>MNFPQLSKEVAEDEAEVILHTSQGDIRIKLFPKLAPLAVENFLTHAKEGYYNGITFHRVIDGFMVQTGDPKGDGTGGQSIWHDKDKTKDKGTGFKNEITPYLYNIRGALAMANTGQPNTNGSQFFINQNSTDTSSKLPTSKYPQKIIEAYKEGGNPSLDGKHPVFGQVIGGMDVVDKIAKAEKDEKDKPTTAITIDSIEVVKDYDFKSENLYFQ[10x]

Here, we solved the protein structures of two secreted parvulin and two secreted cyclophilin-like peptidyl-prolyl isomerase (PPIase) ATP-independent chaperones found in gram-positive streptococcal species. Two types of ATP-independent extracellular PPIases exist in pathogenic streptococci: the parvulin and cyclophilin families. Unlike cytoplasmic PPIases, extracellular PPIases have canonical secretion signal peptides that allow for their translocation across the cell membrane via the Sec pathway. These chaperones are lipidated to the outer leaflet of the membrane and function in the space between the bacterial membrane and cell wall.

In contrast, S. pneumoniae SlrA (SpnSlrA) is a functional PPIase and, like SpnPrsA, is also critical for the colonization of the upper airways as well as for invasive disease. We then solved the crystal structures of SlrA homologs from S. pneumoniae (SpnSlrA) and S. pyogenes (SpyPpiA) to 1.88 Å and 1.28 Å resolution, respectively, using single-wavelength anomalous diffraction (SAD) data from selenomethionine derivatized crystals. Models for two chains (A, D) contain all residues of the recombinant protein: an N-terminal methionine, residues 61–267 of SpnSlrA, and six residues of the fused C-terminal His-tag. For the remaining eight chains, the electron density maps had insufficient quality to model the C-terminal residue. The SpnSlrA and SpyPpiA proteins have a canonical cyclophilin fold comprised of eight antiparallel β-strands (SpnSlrA: β1, 72–81; β2, 82–90; β3, 112–120; β4, 121–127; β5, 166–173; β6, 181–188; β7, 221–227; β8, 250–260) that form a β-barrel with two α-helices (SpnSlrA: α1,95–108; α2, 230–240) located at the top and the bottom of the barrel. Both structures also contain extra secondary structural elements adjacent to the β-barrel composed of residues 189–212 (η2, 193–195; η3, 203–211; η4, 215–217). To gain further insights into these novel structured appendages/insertions, we utilized AlphaFold3 (46) to model our solved SpnSlrA protein structure and a known tetrapeptide substrate (amino acids AAPF) of the human cyclophilin A. The predicted interaction revealed a model where the appendages interact with the AAPF substrate in a dynamic fashion, suggesting that these appendages may aid in substrate recognition or activity. Interestingly, in SpnSlrA, Phe184 at the base of the S1′ pocket and His221 at the side of the S1′ pocket are identical to hCypA residues, but both are replaced by Tyr in SpyPpiA. Using affinity isothermal titration calorimetry (ITC), we determined that SpnSlrA and SpyPpiA bind to CsA with a dissociation constants (Kd) of 122.4 ± 41.4 nM and 365.7 ± 102.1 nM, respectively.> RVADTVGTGPTNSEAIPALTAAETGHTSQVVPGDTMQTRHVKNYHSRSESTIENFLCRSACVYFTEYKNSGAKRYAEWVLTPRQAAQLRRKLEFFTYVRFDLELTFVITSTQQPSTTQNQDAQILTHQIMYVPPGGPVPDKVDSYVWQTSTNPSVFWTEGNAPPRMSIPFLSIGNAYSNFYDGWSEFSRNGVYGINTLNNMGTLYARHVNAGSTGPIKSTIRIYFKPKHVKAWIPRPPRLCQYEKAKNVNFQPSGVTTTRQSITTMTNT;> SDRARSITLGNSTITTQECANVVVGYGVWPDYLKDSEATAEDQPTQPDVATCRFYTLDSVQWQKTSPGWWWKLPDALSNLGLFGQNMQYHYLGRTGYTVHVQCNASKFHQGCLLVVCVPEAEMGCATLDNTPSSAELLGGDTAKEFADKPVASGSNKLVQRVVYNAGMGVGVGNLTIFPHQWINLRTNNSATIVMPYTNSVPMDNMFRHNNVTLMVIPFVPLDYCPGSTTYVPITVTIAPMCAEYNGLRLAG;> GLPTMNTPGSCQFLTSDDFQSPSAMPQYDVTPEMRIPGEVKNLMEIAEVDSVVPVQNVGEKVNSMEAYQIPVRSNEGSGTQVFGFPLQPGYSSVFSRTLLGEILNYYTHWSGSIKLTFMFCGSAMATGKFLLAYSPPGAGAPTKRVDAMLGTHVIWDVGLQSSCVL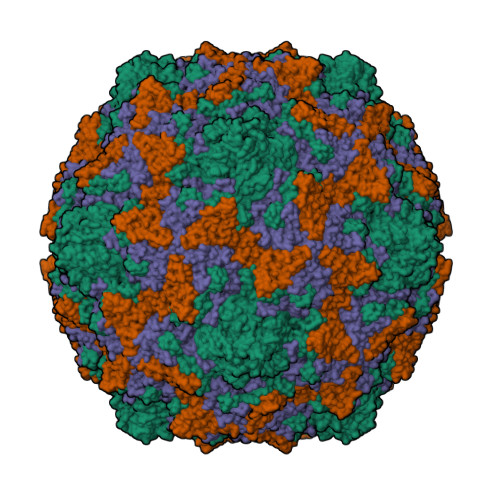CIPWISQTHYRFVASDEYTAGGFITCWYQTNIVVPADAQSSCYIMCFVSACNDFSVRLLKDTPFISQQNFF;> GAQVSTQKTGAHETRLNASGNSIIHYTNINYYKDAASNSANRQDFTQDPGKFTEPVKDIMIKSLPALN>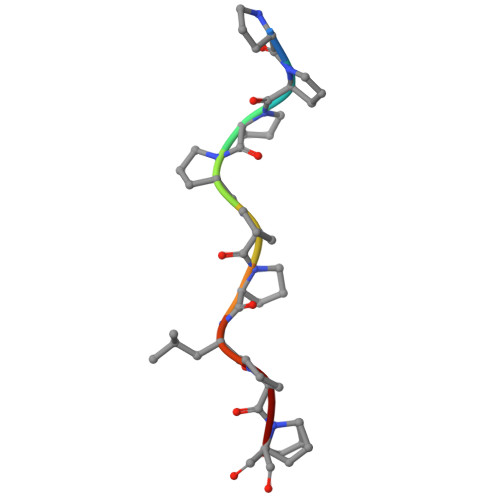 PPPPPPLPP> SDDFLWFEGIAFPTMGFRSETLRKVRDEFVIRDEDVIILTYPKSGTNWLAE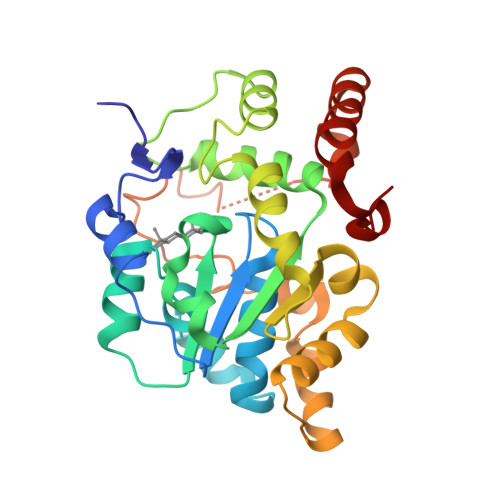ILCLMHSKGDAKWIQSVPIWERSPWVESEIGYTALSETESPRLFSSHLPIQLFPKSFFSSKAKVIYLMRNPRDVLVSGYFFWKNWKFIKKPKSWEEYFEWFCQGTVLYGSWFDHIHGWMPMREEKNFLLLSYEELKQDTGRTIEKICQFLGKTLEPEELNLILKNSSFQSMKENKMSNYSLLSVDYVVDKTQLLRKGVSGDWKNHFTVAQAEDFDKLFQEKMADLPRELFPWE>[2x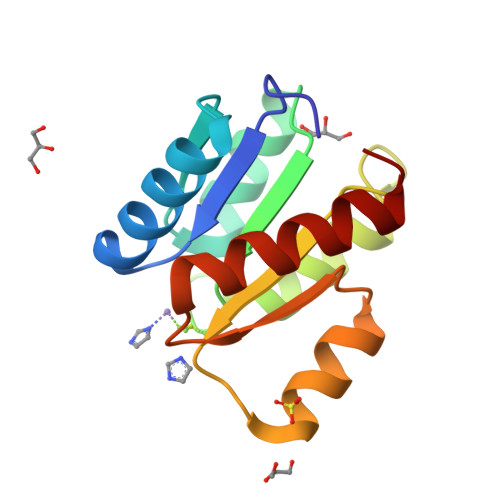]ADKELKFLVVDDQSTMRRIVRNLLKELGFNNVEEAEDGVDALNKLQAGGYGFVISDWKMPNMDGLELLKTIRADGAMSALPVLMVTAYAKKENIIAAAQAGASGYVVKPFTAATLEEKLNKIFEKLGM> MSQRIIQPSASDQQFPGKSDGYEYTVGPKQAITSEASTTYYISRIYSESLLFKRQEASLSAMAFLFQEMISQLHRTCKTAGDFETKLSDYGHNIGIRLLELLNFRASSSPSSLPRASAFLSQNESSSKLSNASNSPGMLANSSTATSASANERLQEKQTESLSNYITKMRRRDLKILDILQFIHGTLWSYLFNHVSDDLVKSSERDNEYMIVDNFPTLTQFIPGENVSCEYFVCGIIKGFLFNAGFPCGVTAHRM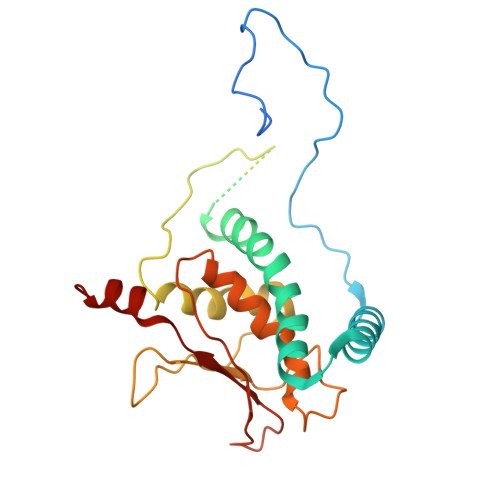PQGGHSQRTVYLIQFDRQVLDREGLRFG> YSPTFNVAHILAFFFLFLHIPF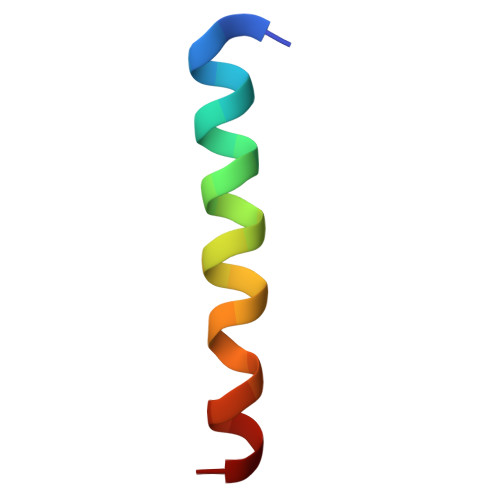YFV> MAQQGVFTLPANTSFGVTA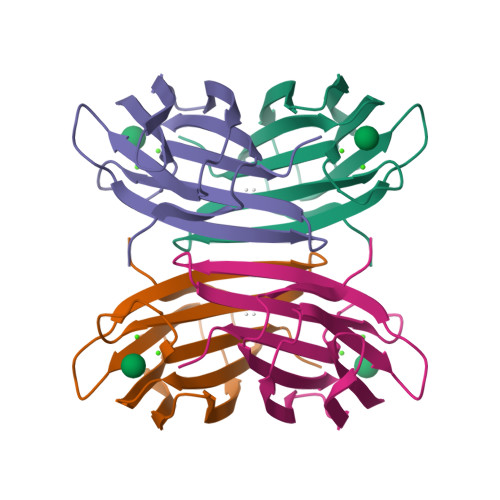FANAANTQTIQVLVDNVVKATFTGSGTSDKLLGSQVLNSGSGAIKIQVSVNGKPSDLVSNQTILANKLNFAMVGSEDGTDNDYNDGIAVLNWPLG> ATQRKGTDEIYGLGSLPSAGPGRWEYLANPGNWHPERRKLHEKLLDQARSSALTLAESLESDGCQPTLFALRGNTATGKTRIATKKIPVLAAALKKTAGKGCVNPDVFKSSLAKSETGAKIFSSAQVHSESSFLADRFEGGLRSQKTGSGAIASIVVDKRLSREYEIDSYIQLAKETGRKVELCDIDAPLENSLVGVLQRKPEGEDPRPPYPVVSSGFVAVRSNRMYVIDRFIADPSLGNYRLFGTAEDGEK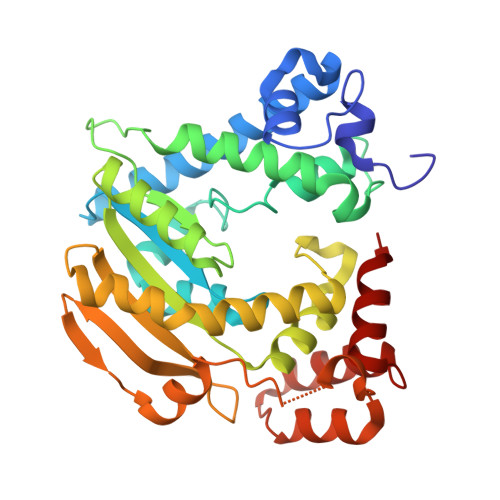VMVASVIGGEFSVENAELYEKITSPQLSVTGDLADKVIDKELIDRLENNIADPERAAKTRAALEKYSGKSWSAALAAHSELI>GSHQKVALHPHDLDERIPGLADLHNQTLGDPQITIVIIDGDPDYTLSCFEGAEVSKVFPYWHEPAEPITPEDYAAFQSIRDQGLKGKEKEEALEAVIPDTKDRIVLNDHACHVTSTIVGQEHSPVFGIAPNCRVINMPQDAVIRGNYDDVMSPLNLARAIDLALELGANIIHCAFCRPTQTSEGEEILVQAIKKCQDNNVLIVSPTGNNSNESWCLPAVLPGTLAVGAAKVDGTPCHFSNWGGNNTKEGILAPGEEILGAQPCTEEPVRLTGTSMAAPVMTGISALLMSLQVQQGKPVDAEAVR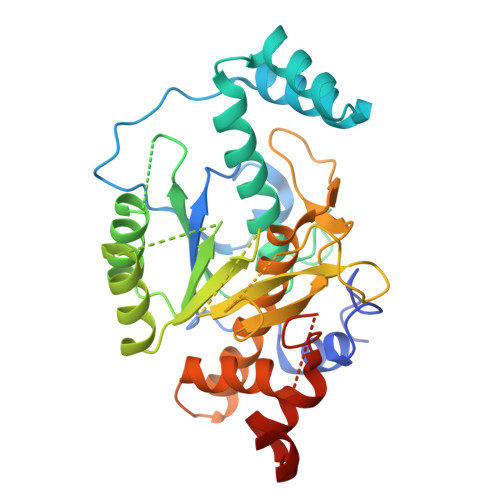TALLKTAIPCDPEVVEEPERCLRGFVNIPGAMKVLFGQPSVTVSFAGGQATRT[2x]> MDKDCEMKRTTLDSPLGKLELSGCEQGLHEIKLLGKGTSAADAV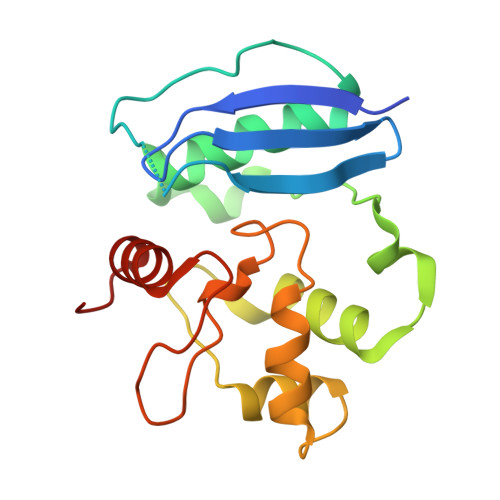EVPAPAAVLGGPEPLMQCTAWLNAYFHQPEAIEEFPVPALHHPVFQQESFTRQVLWKLLKVVKFGEVISYQQLAALAGNPKAARAVGGAMRGNPVPILIPCHRVVCSSGAVGNYSGGLAVKEWLLAHEGHRL> VRAPALSNPRGRIHCRLVAKKELSRDVRLFRFSLPSPDQVLGLPIGKHIFVCATIEGKLCMRAYTPTSMVDEIGHFDLLVKVYFKNEHPKFPNGGLMTQYLDSLPVGSYIDVKGPLGHVEYTGRGSFVINGKQRNARRLAMICGGSGITPMYQIIQAVLRDQPEDHTEMHLVYANRTEDDILLRDELDRWAAE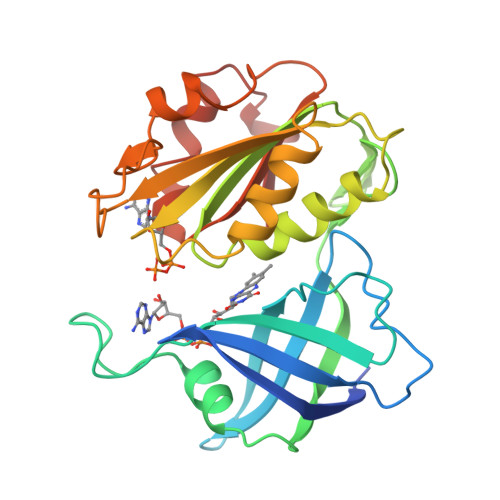YPDRLKVWYVIDQVKRPEEGWKYSVGFVTEAVLREHVPEGGDDTLALACGPPPMIQFAISPNLEKMKYDMANSFVVF The C-ring is tightly attached to the MS-ring, which consists of ~34 FliF molecules with two transmembrane helices. FliF contains three ring-building motifs (RBM1, RBM2, and RBM3) and β-collar in the periplasmic region between the two transmembrane helices. Among these motifs, RBM3–β-collar forms an S-ring on the distal side of the cytoplasm within the MS-ring. We performed single-particle cryo-EM of the purified MS-ring formed by FliFG fusion proteins with the FliG-G214S mutation and determined the near-atomic resolution structure of the Vibrio S-ring.

A total of 228,461 particle images extracted from 5,962 cryo-EM micrographs were analyzed. They were separated into two classes in the 2D class averages, with them showing either 35- or 34-fold rotational symmetry on the S-ring. Because the MS-ring in the native flagellar motor is thought to comprise 34 FliF subunits, it is inferred that the 34-fold rotational symmetry structure reflects the native S-ring structure, whereas the 35-fold rotational symmetry structure is an artificial structure induced by the overexpression of FliFG fusion proteins alone. Consequently, we built the atomic model of the S-ring part (RBM3–β-collar) at 3.23 and 3.33 Å resolutions from the maps of both classes after C35 and C34 rotational symmetry corrections, respectively. The monomeric structures in the S-ring part from the 35- and 34-mer structures are almost identical (RMSD = 0.286 Å). Our S-ring structures are composed of 34 or 35 molecules of the FliFG fusion protein. Their diameters differ: the outer and inner diameters are about 26.0 nm and 9.6 nm, respectively, in the 35-mer ring, and about 25.2 nm and 9.4 nm, respectively, in the 34-mer ring. In our two S-ring structures, the 34-mer structure should reflect the native S-ring structure, since the in situ MS-ring is a 34-mer of FliF. We compared the Vibrio S-ring FliF 34-mer structure with three previously reported Salmonella S-ring FliF 34-mer structures where a notable difference is the tilt angle of the RBM3 domain. When measuring the α1 helix angle from the side-view of the ring, the RBM3 outer part is tilted downwards by 8° in the Vibrio S-ring, whereas it is tilted upwards by 6° or 8° or is nearly horizontal in the Salmonella S-ring. When comparing the β2/β5 sheet angles, they all exhibited a similar angle (55°) when viewed from the outside of the ring, whereas the angle is smallest in the Vibrio S-ring (58°) compared with the Salmonella S-ring (64°–68°) when viewed from the side. When focusing on the subunit interface of the RBM3 during ring formation, interaction was facilitated by two sites: an electrostatic interaction between E270 and K276 and a hydrophobic interaction between A399, V429, and L447 in the Vibrio S-ring.

>[34x]MNHKVHHHHHHIEGRHMADKSTDLTVTEGGSDGALVASSDVDVESQNPDLEERSASKFDMAVGDLDLLRQVVLVLSISICVALIVMLFFWVKEPEMRPLGAYETEELIPVLDYLDQQKINYKLDGNTISVESSEYNSIKLGMVRSGVNQATEAGDDILLQDMGFGVSQRLEQERLKLSRERQLAQAIEEMKQVRKARVLLALPKHSVFVRHNQEASASVFLTLSTGTNLKQQEVDSIVDMVASAVPGMKTSRITVTDQHGRLLSSGSQDPASAARRKEQELERSQEQALREKIDSVLLPILGYGNYTAQVDIQMDFSAVEQTRKRFDPNTPATRSEYALEDYNNGNMVAGIPGALSNQPPADASIPQDVAQMKDGSVMGQGSVRKESTRNFELDTTISHERKQTGTVARQTVSVAIKDRRQVNPDTGEVTYTPMSESEINAIRQVLIGTVGFDQGRGDLLNVLSVKFAEPEAEQLEEPPIWEHPNFSDWVRWFASALVIIVVVLVLVRPAMKKLLNPTSDDEDEMYGPDGLPIGADGETSLIGSDIESSELFEFGSSIDLPNLHKDEDVLKAVRALVANEPELAAQVVKNWMNDMANDIVPQDDNAAGMPVELDVSTITGEEKAAILLLSLNEQDAAGIIRHLEPKQVQRVGSAMAKAKDLSQDKVSAVHRAFLEDIQKYTNIGMGSEDFMRNALVAALGEDKANNLVDQILLGTGSKGLDSLKWMDPRQVASIIVNEHPQIQTIVLSYLEADQSAEILSQFPERVRLDLMMRIANLEEVQPSALAELNEIMEKQFAGQAGAQAAKISGLKAAAEIMNYLDNNVEGLLMEQIRDQDEDMATQIQDLMFVFENLVEVDDQGIQKLLRDVPQDVLQKALKGADDSLREKVFKNMSKRAAEMMRDDIEAMPPVRVADVEAAQKEILAIARRMADAGELMLSGGADEFL Chorismate mutase (CM) and cyclohexadienyl dehydratase (CDT) catalyze two subsequent reactions in the intracellular biosynthesis of l-phenylalanine (Phe). Here, we report the discovery of novel and extremely rare bifunctional fusion enzymes, consisting of fused CM and CDT domains, which are exported from the cytoplasm. In γ-proteobacterial fusion enzymes, the CM domain is N-terminal to the CDT domain, whereas the order is inverted in β-Proteobacteria. The fusion enzymes of Aequoribacter fuscus, Janthinobacterium sp. HH01, and Duganella sacchari were crystallized and their structures refined to 1.6, 1.7, and 2.4 Å resolution, respectively.

To investigate the relative locations of the active sites within a single polypeptide, ∗AfCMCDT, ∗JbCDTCM, and ∗DsCDTCM were crystallized, and their structures solved and refined to 1.6, 1.7, and 2.4 Å resolution, respectively, and Rfree/Rwork values of 24.8/20.5%, 24.3/19.9%, and 25.8/23.0%. Also the structures of ∗DsCDTCM and ∗JbCDTCM are very similar, both overall and in the active site, with r.m.s.d = 1.4 Å (Cα atoms). ∗JbCDTCM and ∗DsCDTCM share the same residues in both CM and CDT active sites. In the two ∗CDTCMs, the distances between CM and CDT active sites are similarly large, measuring approximately 40 Å, thus disfavoring a direct intramolecular transfer of the metabolic intermediate prephenate from the CM to the CDT active site. Whereas ∗AfCMCDT and ∗JbCDTCM crystals contained only one polypeptide chain in the asymmetric unit, the ∗DsCDTCM crystal contained four chains; with head-to-tail dimers (CM-to-CDT) established by crystallographic symmetry. The buried surface area of this ∗DsCDTCM dimer was estimated to be 3070 Å2, with the free energy of dimer dissociation being 5.8 kcal/mol, as calculated using PDBePISA. The dimerization interface is mainly lined with hydrophilic and charged residues. The crystal structure of ∗DsCDTCM head-to-tail dimers allowed us to address possible intermolecular substrate channeling between domains of different protomers in a protein complex. The active sites of the CM and CDT domains of the two individual chains are separated by a substantial distance of about 40 Å and open toward opposite directions. An ATPase and another solute-binding protein are encoded directly downstream of the genes for ∗TaCMCDT and ∗TvCMCDT, whereas for ∗SbCMCDT and ∗SpCMCDT genes, no flanking coding regions with the same orientation were found. Interestingly, an intramembrane protease and an AI-2E family transporter are encoded by the two genes in the same direction and directly upstream of the one for ∗DsCDTCM, which suggests a role in signal recognition.

>[4x]MKRLLLSTLLVTALASAHAGRLEEIHARGVLRVGSTGDYKPFSYRAGANDFIGLDVEQAGELARAMGVKLEIVPTSWPTLMTDFGADKFDIVLSGVSVTAERQQQALFSVSYLRDGKTPITRCENQLRFQTLEQINQPAVRLIVNPGGTNERFARAHAPHAQLTVYPDNVTIFGQIVSGAADLMMTDAIETRLQQRLHPELCAVHPDAPFDTAEKAILLPRDAELKIYVDTWLQQRISSGGLQKSFDRWLDYPWALEPLRQAIDERLLLAEAVARAKWNVQAPIEDLPREAQVIAAAVQQGRTLGLPDAWVAAVFKAQIEASKTVQRELYAKWKAQQAGHFDDAPDLANTIRPQLDRITTQLLRAMADNQATLKDTARLIRPLEAAALSPAAAAQALAPLSAHVVVRFLEHHHHHH>[4x]MSSNAQVRPPLPPFTRESAIEKIRLAEDGWNSRDPE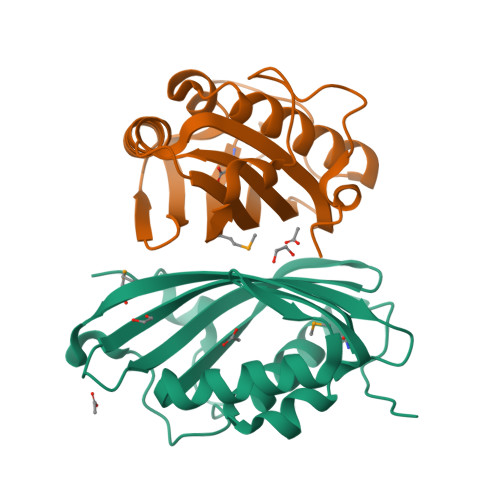RVSLAYTLDTQWRNRAEFAHNREEAKAFLTRKWAKELDYRLIKELWAFTDNRIAVRYAYEWHDDSGNWFRSYGNENWEFDEQGLMARRFACINDMPIKAQERKFHWPLGRRPDDHPGLSELGLEHHHHHH> KETAAAKFERQHMDSSTSAAS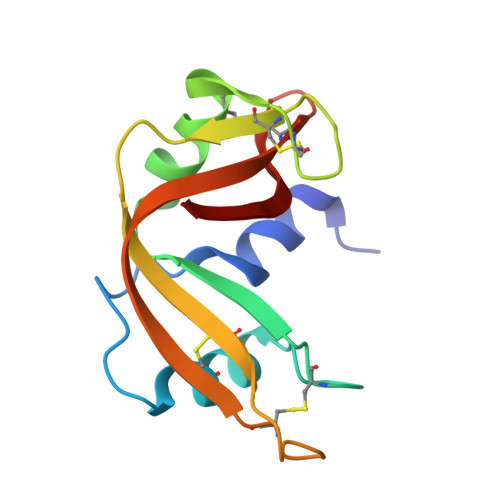SSNYCNQMMKSRNLTKDRCKPVNTFVHESLADVQAVCSQKNVACKNGQTNCYQSYSTMSITDCRETGSSKGPNCAYKTTQANKHIIVACEGNPYVPVHFDASV>[2x]RSGAPGDAALPEPNIFLIFSHGLQGCLEAQGGQVRVTPACNTSLPAQRWKWVSRNRLFNLGTMQCLGTGWPGTNTTASLGMYECDREALNLRWHCRTLGDQLSLLLGARTSNISKPGTLERGDQTRSGQWRIYGSEEDLCALPYHEVYTIQGNSHGKPCTIPFKYDNQWFHGCTSTGREDGHLWCATTQDYGKDERWGFCPIKSND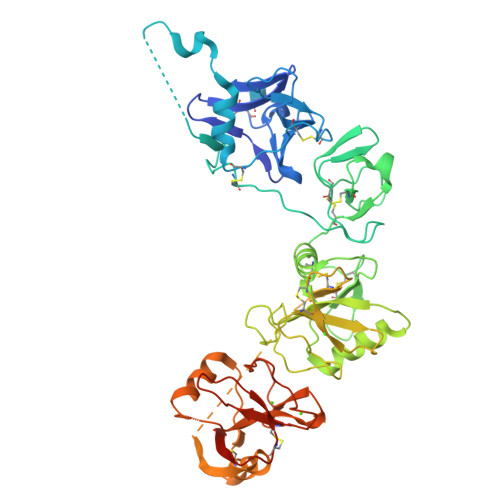CETFWDKDQLTDSCYQFNFQSTLSWREAWASCEQQGADLLSITEIHEQTYINGLLTGYSSTLWIGLNDLDTSGGWQWSDNSPLKYLNWESDQPDNPSEENCGVIRTESSGGWQNRDCSIALPYVCKKKPNATAEPTPPDRWANVKVECEPSWQPFQGHCYRLQAEKRSWQESKKACLRGGGDLVSIHSMAELEFITKQIKQEVEELWIGLNDLKLQMNFEWSDGSLVSFTHWHPFEPNNFRDSLEDCVTIWGPEGRWNDSPCNQSLPSICKKAGQLTRTGHHHHHH> GPDSMKETPLSNCERRFLLRAIEEKKRLDGRQTYDYRNIRISFGTDYGCCIVELGKTRVLGQVSCELVSPKLNRATEGILFFNLELSQMAAPAFEPGRQSDLLVKLNRLMERCLRNSKCIDTESLCVVAGEKVWQIRVDLHLLNHDGNIIDAASIAAIVALCHFRRPDVSVQGDEVTLYTPEERDPVPLSIHHMPICVSFAFFQQGTYLLVDPNEREERVMDGLLVIAMNKHREICTIQSSGGIMLLKDQVLRCSKIAGVKVAEITELILKALENDQKVRKEGGKFGFAESIANQRITAFKMEKAPIDTSDVEEKAEEIIAEAEPPSEVVSTPVLWTPGTAQIGEGVENSWGDLEDSEKEDDEGGGDQAIILDGIKMDTGVEVSDIGSQDAPIILSDSEEEEMIILEPDKNPKKIRTQTTSAKQEKAPSKKPVKRRKKKRAAN;> GPDSMAGLELLSDQGYRVDGRRAGELRKIQARMGVFAQADGSAYIEQGNTKALAVVYGPHEIRGSRARALPDRALVNCQYSSATFSTGERKRRPHGDRKSCEMGLQLRQTFEAAILTQLHPRSQIDIYVQVLQADGGTYAACVNAATLAVLDAGIPMRDFVCACSAGFVDGTALADLSHVEEAAGGPQLALALLPASGQIALLEMDARLHEDHLERVLEAAAQAARDVHTLLDRVVRQHVREASILLGD;> RSMAAGFKTVEPLEYYRRFLKENCRPDGRELGEFRTTTVNIGSISTADGSALVKLGNTTVICGVKAEFAAPSTDAPDKGYVVPNVDLPPLCSSRFRSGPPGEEAQVASQFIADVIENSQIIQKEDLCISPGKLVWVLYCDLICLDYDGNILDACTFALLAALKNVQLP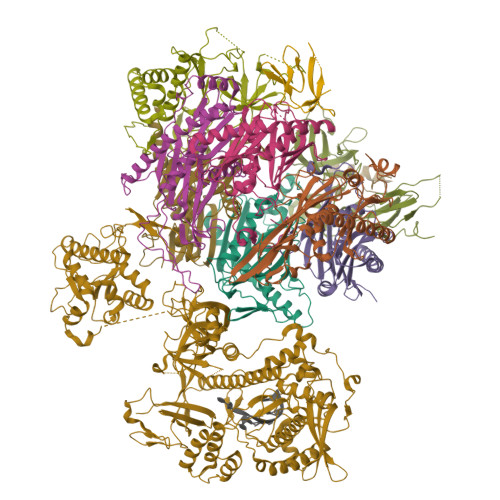EVTINEETALAEVNLKKKSYLNIRTHPVATSFAVFDDTLLIVDPTGEEEHLATGTLTIVMDEEGKLCCLHKPGGSGLTGAKLQDCMSRAVTRHKEVKKLMDEVIKSMKPK;> RSMEEETHTDAKIRAENGTGSSPRGPGCSLRHFACEQNLLSRPDGSASFLQGDTSVLAGVYGPAEVKVSKEIFNKATLEVILRPKIGLPGVAEKSRERLIRNTCEAVVLGTLHPRTSITVVLQVVSDAGSLLACCLNAACMALVDAGVPMRALFCGVACALDSDGTLVLDPTSKQEKEARAVLTFALDSVERKLLMSSTKGLYSDTELQQCLAAAQAASQHVFRFYRESLQRRYSKS;> GPDSMASVTLSEAEKVYIVHGVQEDLRVDGRGCEDYRCVEVETDVVSNTSGSARVKLGHTDILVGVKAEMGTPKLEKPNEGYLEFFVDCSASATPEFEGRGGDDLGTEIANTLYRIFNNKSSVDLKTLCISPREHCWVLYVDVLLLECGGNLFDAISIAVKAALFNTRIPRVRVLEDEEGSKDIELSDDPYDCIRLSVENVPCIVTLCKIGYRHVVDATLQEEACSLASLLVSVTSKGVVTCMRKVGKGSLDPESIFEMMETGKRVGKVLHASLQSVVHKEESLGPKRQKVGFLG;> GPDSMPGDHRRIRGPEESQPPQLYAADEEEAPGTRDPTRLRPVYARAGLLSQAKGSAYLEAGGTKVLCAVSGPRQAEGGERGGGPAGAGGEAPAALRGRLLCDFRRAPFAGRRRRAPPGGCEERELALALQEALEPAVRLGRYPRAQLEVSALLLEDGGSALAAALTAAALALADAGVEMYDLVVGCGLSLAPGPAPTWLLDPTRLEEERAAAGLTVALMPVLNQVAGLLGSGEGGLTESWAEAVRLGLEGCQRLYPVLQQSLVRAARRRGAAAQP;> GSGSGSGSGSGSGSGSGSMAEPASVAAESLAGSRARAARTVLGQVVLPGEELLLPEQEDAEGPGGAVERPLSLNARACSRVRVVCGPGLRRCGDRLLVTKCGRLRHKEPGSGSGGGVYWVDSQQKRYVPVKGDHVIGIVTAKSGDIFKVDVGGSEPASLSYLSFEGATKRNRPNVQVGDLIYGQFVVANKDMEPEMVCIDSCGRANGMGVIGQDGLLFKVTLGLIRKLLAPDCEIIQEVGKLYPLEIVFGMNGRIWVKAKTIQQTLILANILEACEHMTSDQRKQIFSRLAES;> GPDSMAMEMRLPVARKPLSERLGRDTKKHLVVPGDTITTDTGFMRGHGTYMGEEKLIASVAGSVERVNKLICVKALKTRYIGEVGDIVVGRITEVQQKRWKVETNSRLDSVLLLSSMNLPGGELRRRSAEDELAMRGFLQEGDLISAEVQAVFSDGAVSLHTRSLKYGKLGQGVLVQVSPSLVKRQKTHFHDLPCGASVILGNNGFIWIYPTPEHKEEEAGGFIANLEPVSLADREVISRLRNCIISLVTQRMMLYDTSILYCYEASLPHQIKDILKPEIMEEIVMETRQRLLEQEG;> GPDSMAPPVRYCIPGERLCNLEEGSPGSGTYTRHGYIFSSLAGCLMKSSENGALPVVSVVRETESQLLPDVGAIVTCKVSSINSRFAKVHILYVGSMPLKNSFRGTIRKEDVRATEKDKVEIYKSFRPGDIVLAKVISLGDAQSNYLLTTAENELGVVVAHSESGIQMVPISWCEMQCPKTHTKEFRKVARVQPEFLQT;> GPDSMLKSKTFLKKTRAGGVMKIVREHYLRDDIGCGAPGCAACGGAHEGPALEPQPQDPASSVCPQPHYLLPDTNVLLHQIDVLEDPAIRNVIVLQTVLQEVRNRSAPVYKRIRDVTNNQEKHFYTFTNEHHRETYVEQEQGENANDRNNRAIRVAAKWYNEHLKKMSADNQLQVIFITNDRRNKEKAIEEGIPAFTCEEYVKSLTANPELIDRLACLSEEGNEIESGKIIFSEHLPLSKLQQGIKSGTYLQGTFRASRENYLEATVWIHGDNEENKEIILQGLKHLNRAVHEDIVAVELLPKSQWVAPSSVVLHDEGQNEEDVEKEEETERMLKTAVSEKMLKPTGRVVGIIKRNWRPYCGMLSKSDIKESRRHLFTPADKRIPRIRIETRQASTLEGRRIIVAIDGWPRNSRYPNGHFVRNLGDVGEKETETEVLLLEHDVPHQPFSQAVLSFLPKMPWSITEKDMKNREDLRHLCICSVDPPGCTDINDALHCRELENGNLEVGVHIADVSHFIRPGNALDQESARRGTTVYLCEKRIDMVPELLSSNLCSLKCDVDRLAFSCIWEMNHNAEILKTKFTKSVINSKASLTYAEAQLRIDSANMNDDITTSLRGLNKLAKILKKRRIEKGALTLSSPEVRFHMDSETHDPIDLQTKELRETNSMVEEFMLLANISVAKKIHEEFSEHALLRKHPAPPPSNYEILVKAARSRNLEIKTDTAKSLAESLDQAESPTFPYLNTLLRILATRCMMQAVYFCSGMDNDFHHYGLASPIYTHFTSPIRRYADVIVHRLLAVAIGADCTYPELTDKHKLADICKNLNFRHKMAQYAQRASVAFHTQLFFKSKGIVSEEAYILFVRKNAIVVLIPKYGLEGTVFFEEKDKPNPQLIYDDEIPSLKIEDTVFHVFDKVKVKIMLDSSNLQHQKIRMSLVEPQIPGISIPTDTSNMDLNGPKKKKMKLGK;> GPDSASMAAERKTKLSKNLLRMKFMQRGLDSETKKQLEEEEKKIISEEHWYLDLPELKEKESFIIEEQSFLLCEDLLYGRMSFRGFNPEVEKLMLQMNAKHKAEEVEDETVELDVSDEEMARRYETLVGTIGKKFARKRDHANYEEDENGDITPIKAKKMFLKPQD L-THREONOHYDROXAMATE 4-PHOSPHATE | C4 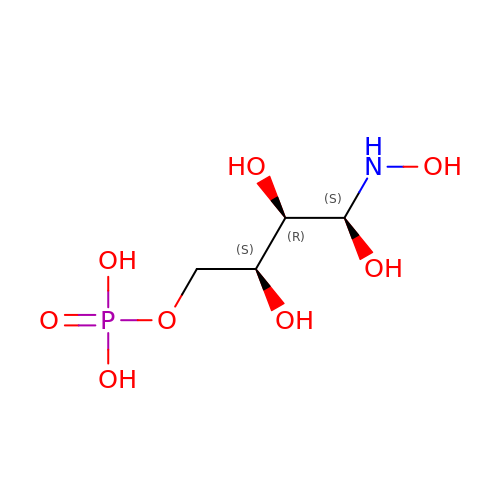H12 N O8 P | CSVKNYIFCYRDJM-NUNKFHFFSA-N N-[4-[(3-cyano-4-naphthalen-2-yloxy-phenyl)sulfamoyl]phenyl]ethanamide 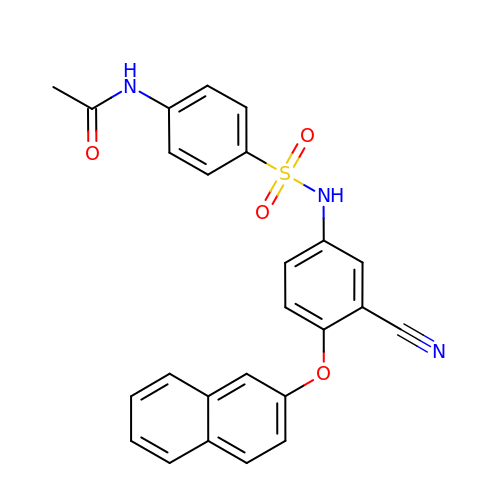| C25 H19 N3 O4 S | XLRISFAORWYVBT-UHFFFAOYSA-N>[2x]MSLFSERLKEI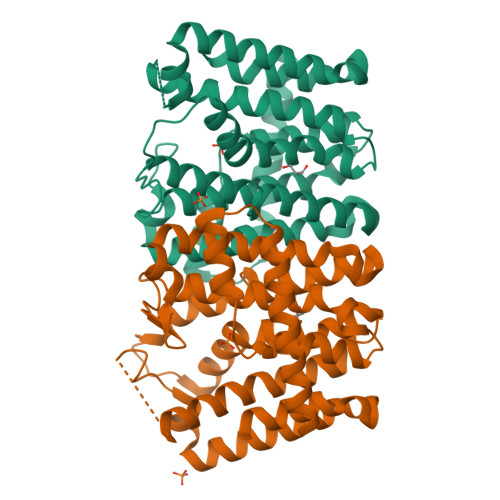QDAVETAMAAAIGRLPAGDLRDAMAYAAQGGKRLRAFLAIESAAIHGISMAQAMPAALAVEALHAYSLVHDDMPCMDNDDLRRGLPTVHKKWDDATAVLAGDALQTLAFELCTDPVLGSAENRVALVAALAQASGAEGMVYGQALDIAAETAAVPLTLDEIIRLQAGKTGALISFAAQAGAILAGADRGPLTAYATALGLAFQIADDILDVEGNEEAAGKRLGKDAEAHKATFVSLLGLAGAKSRAADLVAEAEAALAPYGEAASTLRACARYVIERDKEGHHHHHH> MGKEKTHINIVVIGHVDSGKSTTTGHLIYKCGGIDKRTIEKFEKEAAEMGKGSFKYAWVLDKLKAERERGITIDISLWKFETTKYYITIIDAPGHRDFIKNMITGTSQADCAVLIVAAGVGEFEAGISKNGQTREHALLAYTLGVKQLIVGVNKMDSTEPAYSEKRYDEIVKEVSAYIKKIGYNPATVPFVPISGWHGDNMLEPSPNMPWFKGWKVERKEGNASGVSLLEALDTILPPTRPTDKPLRLPLQDVYKIGGIGTVPVGRVETGILRPGMVVTFAPVNITTEVKSVEMHHEALSEALPGDNVGFNVKNVSVKDIRRGNVCGDSKSDPPQEAAQFTSQVIILNHPGQISAGYSPVIDCHTAHIACKFAELKEKIDRRSGKKLEDNPKSLKSGDAAIVEMVPGKPMCVESFSQYPPLGRFAVRDMRQTVAVGVIKNVEKKSGGAGKVTKSAQKAQKAGK

The dynamic ribosome–translocon complex, which resides at the endoplasmic reticulum (ER) membrane, produces a major fraction of the human proteome. It governs the synthesis, translocation, membrane insertion, N-glycosylation, folding and disulfide-bond formation of nascent proteins. Here we use cryo-electron tomography, extensive classification and molecular modelling to capture snapshots of mRNA translation and protein maturation at the ER membrane at molecular resolution. In sum, we visualize ER-bound polysomes with their coordinated downstream machinery.

We identify a highly abundant classical pre-translocation intermediate with eukaryotic elongation factor 1a (eEF1a) in an extended conformation, suggesting that eEF1a may remain associated with the ribosome after GTP hydrolysis during proofreading. Next, we observe a highly abundant intermediate (33%) that has not been described previously: whereas the tRNA is accommodated in the canonical A-site and the SSU ‘rolls’ into the classical pre-configuration, eEF1a is bound to the ribosome in an extended conformation, which matches crystal structures of purified eEF1A–GDP26 and its bacterial homologue EF-Tu–GDP27. To analyse the pre+ state at higher resolution, we rapidly isolated soluble ribosomes and imaged them with cryo-EM single-particle analysis (SPA). Approximately 30% of particles were in the pre+ state, yielding a focused reconstruction of eEF1a with specific side chains of domain 3 (approximately 3.5 Å resolution) unambiguously identifying eEF1a. In the classical pre+ state, eEF1a domains 1 and 3 interact with the sarcin–ricin loop (SRL) of the 28S rRNA, whereas domain 2 blocks the A/T site and contacts the A-site tRNA. In a model of the human elongation cycle, we propose that the classical pre+ state may follow the decoding state, in which eEF1a still adopts a compact conformation. Although we cannot rule out that other factors observed at this site in situ could have been displaced by eEF1A during the purification, the occurrence of the eEF1A bound classical pre+ state in purified samples indicates the possibility that eEF1a may remain bound to the ribosome during conformational switching to the extended form. The functional relevance of a possible eEF1a-bound classical pre+ state remains to be further investigated with complementary methods.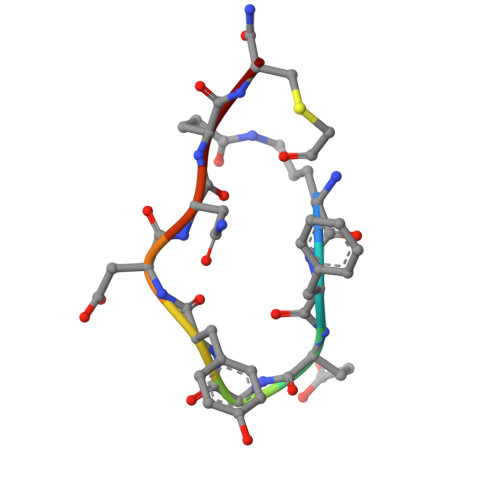> KFEGYDNEX> SAVRLIDLENNASFSKSLNSTTRSHKCTLPIWAGDGEGNVSDSVTLQDVLANDALVEFATDKNGCRFLQEHYPTENDNDVHQKLFRKLVEDRAIFLSLCSNMF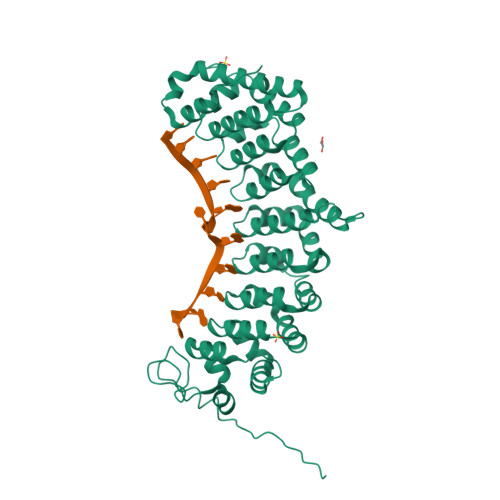GNFFVQRVLECSNTEEQEILTEHLATDLYNLCLDKSACRVIQLAIQKLDVHLATRLSLELRDTHLVRLSIDQNGNHVIQKIVKTLPVSSWTFLVDFFADDDNLIHVCQDKYGCRVIQSTVETLSTDQYAQCYQHRVILLRSLMAGVTRNCTQLASNEFANYVVQHVIKCGDALAVYRDIIIEQCLLQNLLSMSQEKYASHVVEVAFECAPYRLVAEMMNEIFEGYIPHPDTNRDALDILLFHQYGNYVVQQMIQTCVLGQNARDQKQSEMYGMWLEKIHGRVMRNAHRLERFSSGKKIIEALQSMSLY>PSVYDAAAQLTADVKKDLRDSWKVIGSDKKGNGVAFMTTLFADNQETIGYFKRLGDVSQGMANDKLRGHSITLMYALQNFIDQLDNPDDLVCVVEKFAVNHITRKISAAEFGKINGPIKKVLASKNFGDKYANAWAKLVAVVQAAL[2x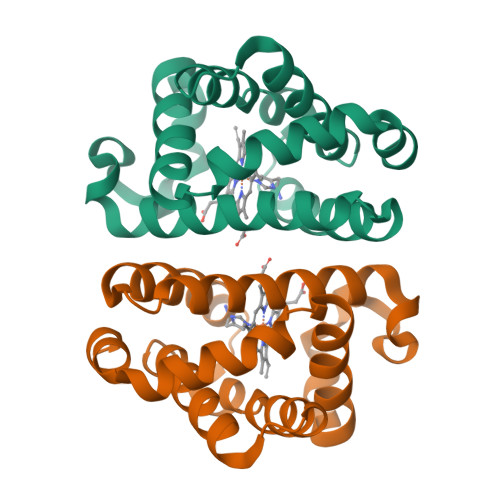]> MEAILSKMKEVVENPNAAVKKYKSETGKKAIGCFPVYCPEEIIHAAGMLPVGIWGGQTELDLAKQYFPAFACSIMQSCLEYGLKGAYDELSGVIIPGMCDTLICLGQNWKSAVPHIKYISLVHPQNRKLEAGVKYLISEYKGVKRELEEICGYEIEEAKIHESIEVYNEHRKTMRDFVEVAYKHSNTIKPSIRSLVIKSGFFMRKEEHTELVKDLIAKLNAMPEEVCSGKKVLLTGILADSKDILDILEDNNISVVADDLAQETRQFRTDVP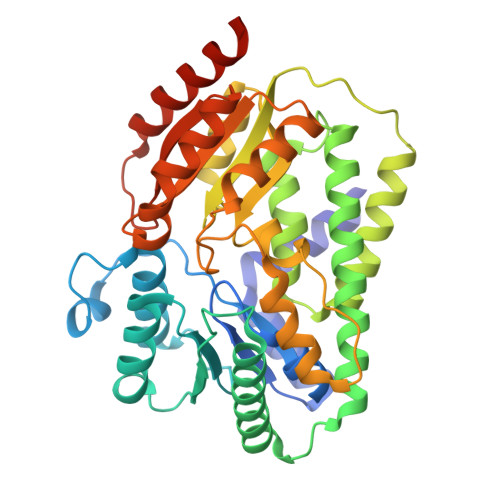AGDDALERLARQWSNIEGCSLAYDPKKKRGSLIVDEVKKKDIDGVIFCMMKFCDPEEYDYPLVRKDIEDSGIPTLYVEIDQQTQNNEQARTRIQTFAEMMSLASAWSHPQFEK> MSLVLNDLLICCRQLEHDRATERKKEVEKFKRLIRDPETIKHLDRHSDSKQGKYLNWDAVFRFLQKYIQKETECLRIAKPNVSASTQASRQKKMQEISSLVKYFIKCANRRAPRLKCQELLNYIMDTVKDSSNGAIYGADCSNILLKDILSVRKYWCEISQQQWLELFSVYFRLYLKPSQ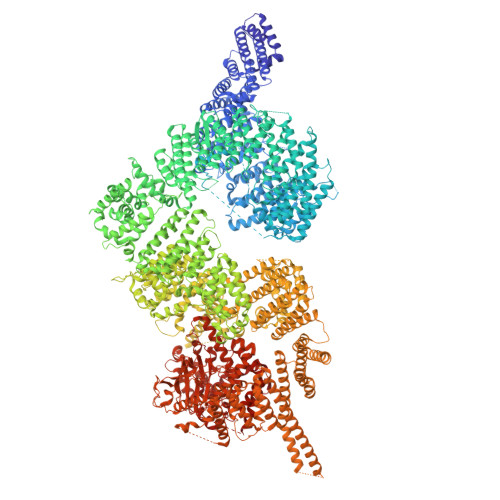DVHRVLVARIIHAVTKGCCSQTDGLNSKFLDFFSKAIQCARQEKSSSGLNHILAALTIFLKTLAVNFRIRVCELGDEILPTLLYIWTQHRLNDSLKEVIIELFQLQIYIHHPKGAKTQEKGAYESTKWRSILYNLYDLLVNEISHIGSRGKYSSGFRNIAVKENLIELMADICHQVFNEDTRSLEISQSYTTTQRESSDYSVPCKRKKIELGWEVIKDHLQKSQNDFDLVPWLQIATQLISKYPASLPNCELSPLLMILSQLLPQQRHGERTPYVLRCLTEVALCQDKRSNLESSQKSDLLKLWNKIWCITFRGISSEQIQAENFGLLGAIIQGSLVEVDREFWKLFTGSACRPSCPAVCCLTLALTTSIVPGTVKMGIEQNMCEVNRSFSLKESIMKWLLFYQLEGDLENSTEVPPILHSNFPHLVLEKILVSLTMKNCKAAMNFFQSVPECEHHQKDKEELSFSEVEELFLQTTFDKMDFLTIVRECGIEKHQSSIGFSVHQNLKESLDRCLLGLSEQLLNNYSSEITNSETLVRCSRLLVGVLGCYCYMGVIAEEEAYKSELFQKAKSLMQCAGESITLFKNKTNEEFRIGSLRNMMQLCTRCLSNCTKKSPNKIASGFFLRLLTSKLMNDIADICKSLASFIKKPFDRGEVESMEDDTNGNLMEVEDQSSMNLFNDYPDSSVSDANEPGESQSTIGAINPLAEEYLSKQDLLFLDMLKFLCLCVTTAQTNTVSFRAADIRRKLLMLIDSSTLEPTKSLHLHMYLMLLKELPGEEYPLPMEDVLELLKPLSNVCSLYRRDQDVCKTILNHVLHVVKNLGQSNMDSENTRDAQGQFLTVIGAFWHLTKERKYIFSVRMALVNCLKTLLEADPYSKWAILNVMGKDFPVNEVFTQFLADNHHQVRMLAAESINRLFQDTKGDSSRLLKALPLKLQQTAFENAYLKAQEGMREMSHSAENPETLDEIYNRKSVLLTLIAVVLSCSPICEKQALFALCKSVKENGLEPHLVKKVLEKVSETFGYRRLEDFMASHLDYLVLEWLNLQDTEYNLSSFPFILLNYTNIEDFYRSCYKVLIPHLVIRSHFDEVKSIANQIQEDWKSLLTDCFPKILVNILPYFAYEGTRDSGMAQQRETATKVYDMLKSENLLGKQIDHLFISNLPEIVVELLMTLHEPANSSASQSTDLCDFSGDLDPAPNPPHFPSHVIKATFAYISNCHKTKLKSILEILSKSPDSYQKILLAICEQAAETNNVYKKHRILKIYHLFVSLLLKDIKSGLGGAWAFVLRDVIYTLIHYINQRPSCIMDVSLRSFSLCCDLLSQVCQTAVTYCKDALENHLHVIVGTLIPLVYEQVEVQKQVLDLLKYLVIDNKDNENLYITIKLLDPFPDHVVFKDLRITQQKIKYSRGPFSLLEEINHFLSVSVYDALPLTRLEGLKDLRRQLELHKDQMVDIMRASQDNPQDGIMVKLVVNLLQLSKMAINHTGEKEVLEAVGSCLGEVGPIDFSTIAIQHSKDASYTKALKLFEDKELQWTFIMLTYLNNTLVEDCVKVRSAAVTCLKNILATKTGHSFWEIYKMTTDPMLAYLQPFRTSRKKFLEVPRFDKENPFEGLDDINLWIPLSENHDIWIKTLTCAFLDSGGTKCEILQLLKPMCEVKTDFCQTVLPYLIHDILLQDTNESWRNLLSTHVQGFFTSCLRHFSQTSRSTTPANLDSESEHFFRCCLDKKSQRTMLAVVDYMRRQKRPSSGTIFNDAFWLDLNYLEVAKVAQSCAAHFTALLYAEIYADKKSMDDQEKRSLAFEEGSQSTTISSLSEKSKEETGISLQDLLLEIYRSIGEPDSLYGCGGGKMLQPITRLRTYEHEAMWGKALVTYDLETAIPSSTRQAGIIQALQNLGLCHILSVYLKGLDYENKDWCPELEELHYQAAWRNMQWDHCTSVSKEVEGTSYHESLYNALQSLRDREFSTFYESLKYARVKEVEEMCKRSLESVYSLYPTLSRLQAIGELESIGELFSRSVTHRQLSEVYIKWQKHSQLLKDSDFSFQEPIMALRTVILEILMEKEMDNSQRECIKDILTKHLVELSILARTFKNTQLPERAIFQIKQYNSVSCGVSEWQLEEAQVFWAKKEQSLALSILKQMIKKLDASCAANNPSLKLTYTECLRVCGNWLAETCLENPAVIMQTYLEKAVEVAGNYDGESSDELRNGKMKAFLSLARFSDTQYQRIENYMKSSEFENKQALLKRAKEEVGLLREHKIQTNRYTVKVQRELELDELALRALKEDRKRFLCKAVENYINCLLSGEEHDMWVFRLCSLWLENSGVSEVNGMMKRDGMKIPTYKFLPLMYQLAARMGTKMMGGLGFHEVLNNLISRISMDHPHHTLFIILALANANRDEFLTKPEVARRSRITKNVPKQSSQLDEDRTEAANRIICTIRSRRPQMVRSVEALCDAYIILANLDATQWKTQRKGINIPADQPITKLKNLEDVVVPTMEIKVDHTGEYGNLVTIQSFKAEFRLAGGVNLPKIIDCVGSDGKERRQLVKGRDDLRQDAVMQQVFQMCNTLLQRNTETRKRKLTICTYKVVPLSQRSGVLEWCTGTVPIGEFLVNNEDGAHKRYRPNDFSAFQCQKKMMEVQKKSFEEKYEVFMDVCQNFQPVFRYFCMEKFLDPAIWFEKRLAYTRSVATSSIVGYILGLGDRHVQNILINEQSAELVHIDLGVAFEQGKILPTPETVPFRLTRDIVDGMGITGVEGVFRRCCEKTMEVMRNSQETLLTIVEVLLYDPLFDWTMNPLKALYLQQRPEDETELHPTLNADDQECKRNLSDIDQSFNKVAERVLMRLQEKLKGVEEGTVLSVGGQVNLLIQQAIDPKNLSRLFPGWKAWV> GADLADRFAELERR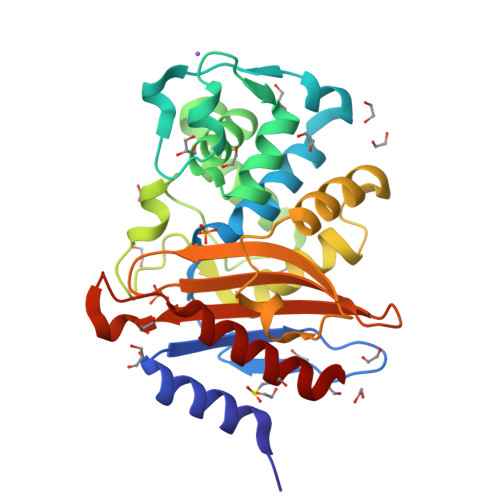YDARLGVYVPATGTTAAIEYRADERFAFCSTFKAPLVAAVLHQNPLTHLDKLITYTSDDIRSISPVAQQHVQTGMTIGQLCDAAIRYSDNTAANLLLADLGGPGGGTAAFTGYLRSLGDTVSRLDAEEPELNRDPPGDERDTTTPHAIALVLQQLVLGNALPPDKRALLTDWMARNTTGAKRIRAGFPADWKVIDKTGTGDYGRANDIAVVWSPTGVPYVVAVMSDRAGGGYDAEPREALLAEAATCVAGVLA>[2x]GSHMSDSNTITSFQVDCYLWHIRKLLSMRDMCDAPFDDRLRADQAALKG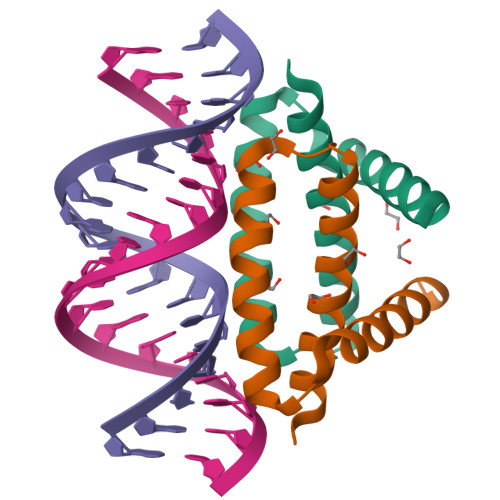RGSTLGLDLRVATMEGKKIVEDILKSET> AQPDPKLDELNKVSDYKSNKGTMGNVMNLYMSPPVEGRGVINSRQFLSHDLIFPIEYKSYNEVKTELENTELANNYKGKKVDIFGVPYFYTCIIPKSEPDINQNFGGCCMYGGLTFNSSENERDKLITVQVTIDNRQSLGFTITTNKNMVTIQELDYKARHWLTKEKKLYEFDGSAFES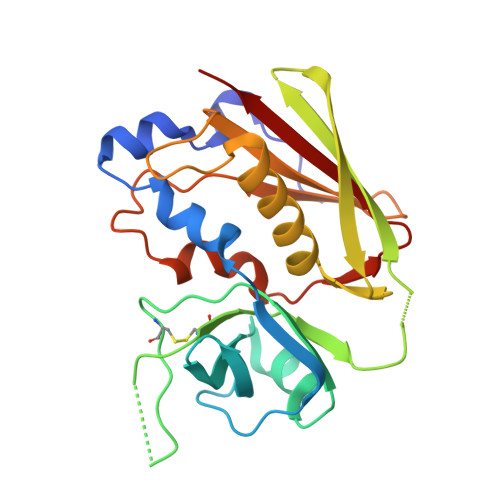GYIKFTEKNNTSFWFDLFPKKELVPFVPYKFLNIYGDNKVVDSKSIKMEVFLNTH>GLVPRGSMIMKDGIYSIIFISNEDSCGEGILIKNGNMITGGDIASVYQGVLSEDEDIILHVHRYNYEI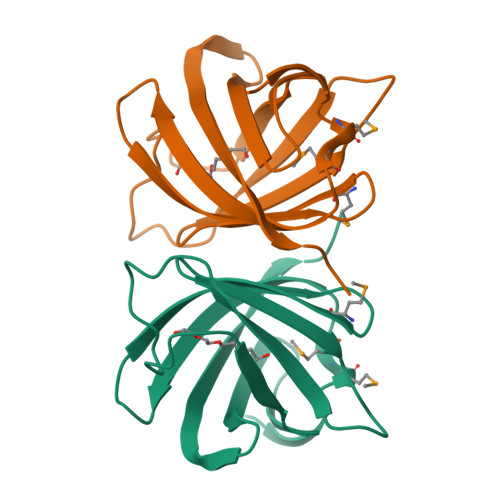PSVLNIEQDYQLVIPKKVLSNDNNLTLHCHVRGNEKLFVDVYAKFIEPLV[2x]> MERAVDARRAIYELWSRTAAAEEHAQFSSDSTSTGEEAAAEAKAAEERSTAVAALLDKYKLDPATPREEDISRGLGDALDRLLLLCVPLSSRHGADLLVKLMQVSAQQGRQFSMRTIQHLFARTSSYAEALAVFYAMRRSNFAMSMEAYHAMLYSLQRLEEEGWAARFHEEFAASKGEAISEQALDFVLRGVDN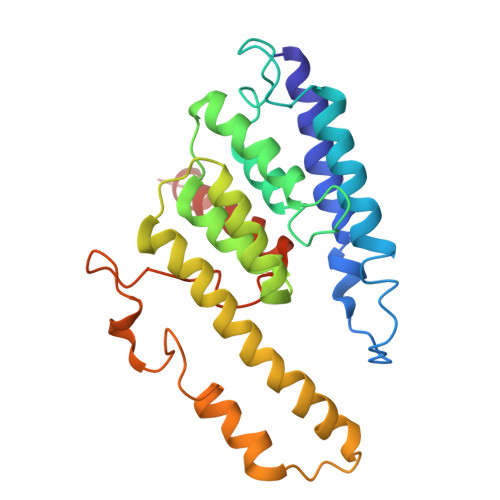QLMPENKPWLGRIMFAEVKDNKATQRQSMASFDAMGKLWVQRYKNGGTAPE>GAMGSRKSKAELQSEERKRIDELIESGKEEGMKIDLIDGKGRGVIATKQFSRGDFVVEYHGDLIEITDAKKREALYAQDPSTGCYMYYFQYLSKTYCVDATRETNRLGRLINHSKCGNCQTKLHDIDGVPHLILIASRDIAAGEELLF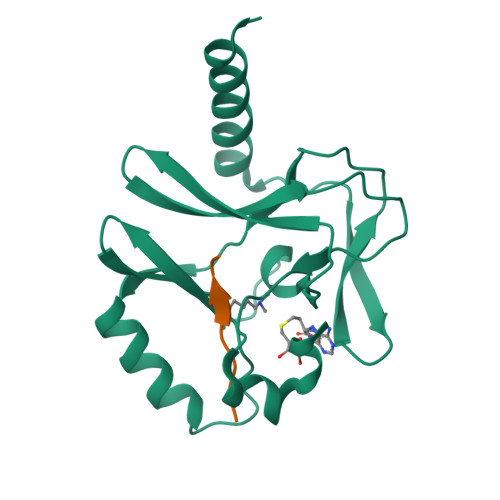DYGDRSKASIEAHPWLKH[4x];>[4x]AKRHRKVLRD> MFYSLMRESKIVIEYDGRGYHFDALSNYDASTSFQEFKTLRRTIHNRTNYADSIINAQDPSSISLAINFSTTLIESNFFDWMGFTREGNSLFLPRNTPNIEPIMFNMYIINHNNSCIYFENCYVSTVDFSLDKSIPILNVGIESGKFSEVSTFRDGYTITQGEVLPYSAPAVYTNSSPLPALISASMSFQQQCSWRE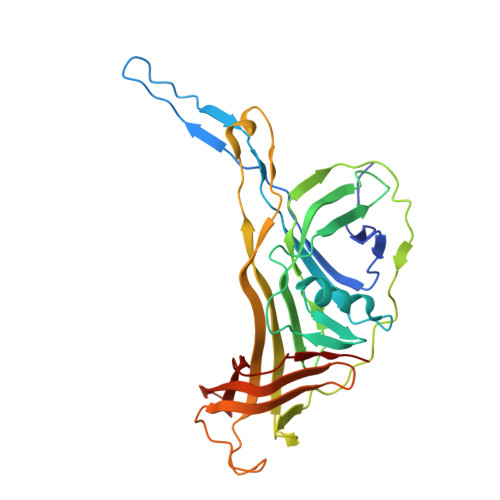DRNIFDINKIYTNKRAYVNEMNASATLAFYYVKRLVGDKFLNLDPETRTPLIIKNKYVSITFPLARISKRLNFSDLYQVEYDVIPTADSDPVEINFFGERK> GFPLITI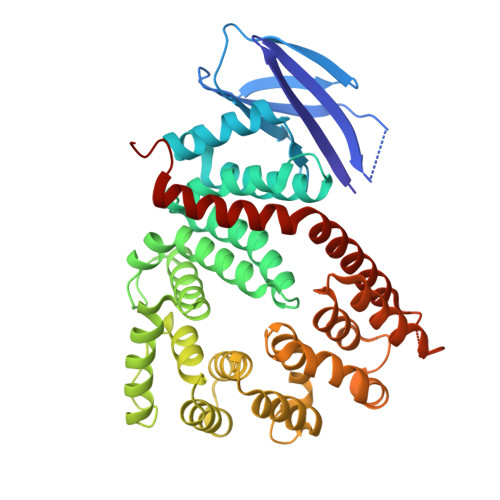TVRGRNVHMKQEHYMKGSDGAPDTGYLWHVPLTFITSKSDMVHRFLLKTKTDVLILPEEVEWIKFNVGMNGYYIVHYEDDGWDSLTGLLKGTHTAVSSNDRASLINNAFQLVSIGKLSIEKALDLSLYLKHETEIMPVFQGLNELIPMYKLMEKRDMNEVETQFKAFLIRLLRDLIDKQTWTDEGSVSERMLRSQLLLLACVHNYQPCVQRAEGYFRKWKESNGNLSLPVDVTLAVFAVGAQSTEGWDFLYSKYQFSLSSTEKSQIEFALCRTQNKEKLQWLLDESFKGDKIKTQEFPQILTLIGRNPVGYPLAWQFLRKNWNKLVQKFELGSSSIAHMVMGTTNQFSTRTRLEEVKGFFSSLKENGSQLRCVQQTIETIEENIGWMDKNFDKIRVWLQSEKLERMIINFEKL> MLKKNETFYTYCSYKKEDGYVRRGLIVLPTLHIAMFAPFLLALLVPFFYKCIRSLHVGWFVFPLPIALFVYFLSYIDDVRNDEVIRATMPWIPSLRISFDAYVDGLSLL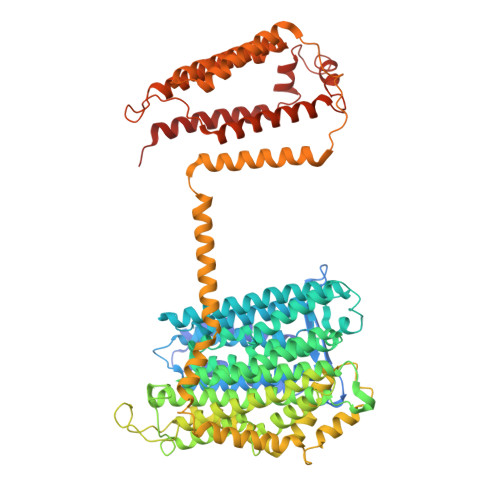FALLITGIGSLVVLYSIYYLQKGKEPLGNFYVYLLLFMGAMLGVVLSDHLIALYMFWELTSISSFLLIAYWFKRDRSRYGAQKSMLITMFGGLLMLGGFVALAIAGGTYNIRELVHTPLTEHPLFIPALVLILFGAFTKSAQFPFYIWLPDAMEAPTPVSAYLHSATMVKAGIYVIARLTPIFAVSSVWVWTVALVGLVTLCWASFLASKQTDLKAILAYSTVSQLGLITSLLGIGGLSFHYDGMGENVFMVAVLAAIFHLFNHATFKGSLFMVVGIVDHETGTRDIRRLGGLMTIMPITFTIALIGSLSMAGLPPFNGFLSKEMFFTAMLRAKDVAGWAVILPVVAWVASIFTFLYSALLVSRTFFGTYKPHVLKKEAHEAPFGMLIAPIVLASLVVFIGFVPNVLSDSVLAPAVYAVLYGLFAPNEALDVHISHWHGFTPELFMTIGVLLFGLVLYRTFPKWKKIYYRLSERMSLNFFYDQSFVWMERGARSFISRVMNGSMRTYLMYIFTSLVALLLFTIGWHEQWHIDLSRLAHVRVYEVVLAIGILAATVTTVIAKSRLTAIVSLGAVGYAVALFFVLFRAPDLALTQLVIETISVALFLLCFYHLPKFTQKQESVRFHLGNALVSLAVGMTMSIIAFLAYAGKHFDSISQYYVDNTYEKAAGKNMVNVILVDFRGFDTLFEICVLAIAALGIYAMVKLRLAKEEER>MKQYLELMQKVLDEGTQKNDRTGTGTLSIFGHQMRFNLQDGFPLVTTKRCHLRSIIHELLWFLQGDTNIAYLHENNVTIWDEWADENGDLGPVYGKQWRAWPTPDGRHIDQITTVLNQLKNDPDSRRIIVSAWNVGELDKMALAPCHAFFQFYVADGKLSCQLYQRSCCVFLGLPFNIASYALLVHMMAQQCDLEVGDFVWTGGDTHLYSNHMDQTHLQLSREPRPLPKLIIKRKPESIFDYRFEDFEIEGYDPHPGIKAPVAI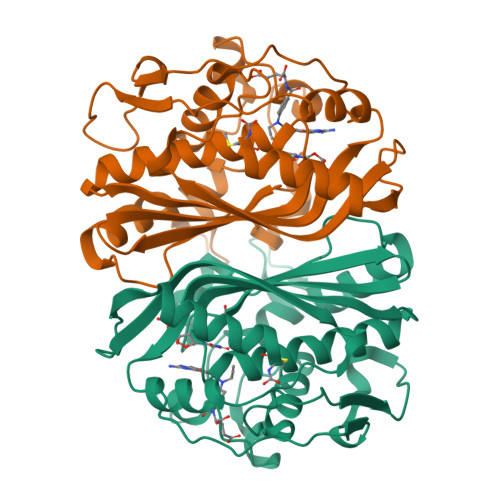[2x]> MGSDKIHHHHHHMKFFSLADEAEFKSIIISKNKAVDVIGSKLGGQVVSFSDEWFASAENLIQPTAPIRDPTRFVHSGAWYDGWETRRHNEMEYDWVIIKMGVAAAHIIGGEIDTAFFNGNHAPFVSIEALYDEGEEGNIVEDDSRWVEIVEKFECGPSQRHLFVRGNGLTKERFTHIKLKMYPDGGIARFRLYGRVVP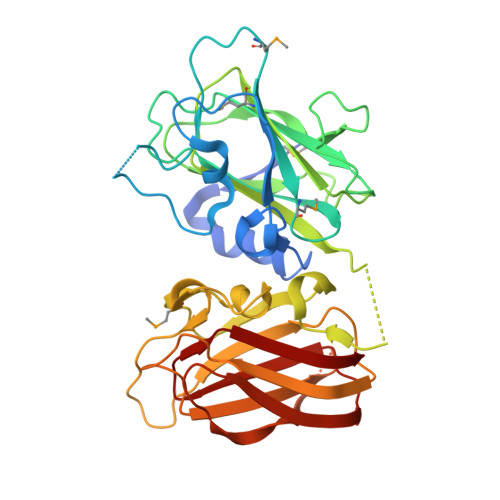PELKTKDHIIDLAYVCNGAVALKYSDQHFGSVDNLLLPGRGHDMSDGWETKRSRQPGHTDWAVIQLGRESSFIEKIIVDTAHFRGNFPQFITVEGCLKESESSENTGEGTWVELVGKSKTGPDKEHVYEIRKSIRVSHVKLTIIPDGGVKRIRVWGY>[4x]GM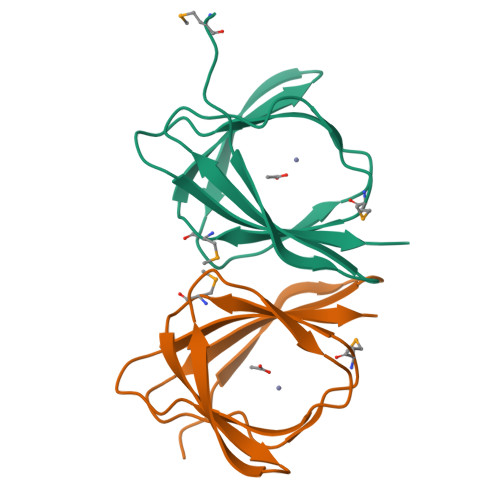KRPGAIPTVQIDNERVKVTEWRFPPGGETGWHRHSMDYVVVPMTTGPLLLETPEGSVTSQLTRGVSYTRPEGVEHNVINPSDTEFVFVEIEIKAA One such potential target is the mycobacterial phosphatidylinositol phosphate synthase (M. tuberculosis PgsA1). PgsA1 catalyzes the conjugation of the 1’ hydroxyl group of D-myo-inositol-3-phosphate (ino-P) with a lipid tail of an acceptor substrate, cytidine diphosphate diacylglycerol (CDP-DAG), forming phosphatidylinositol phosphate (PIP). 1 D-myo-inositol-3-phosphate+CDP-DAG→PIP+CMP 2 PIP→PI+Pi PgsA1 belongs to the class I CDP-alcohol phosphotransferases (CDP-APs), integral membrane proteins that catalyze the formation of a phosphodiester bond to merge a CDP-alcohol and a second alcohol, releasing cytidine monophosphate (CMP). The M. tuberculosis PgsA1 was identified as a promising candidate for drug development, due to its essential role in growth and proliferation of the pathogen and differences between the Eukaryotic and mycobacterial PI biosynthesis pathways.

Here, we present the crystal structure of the full-length M. tuberculosis PgsA1 in absence of metals and substrates (apo) to 2.9 Å resolution and the 1.8 Å resolution structure of the CDP-DAG complex with a di-nuclear catalytic Mg2+ site. The electron density map does not contain any unexplained positive density in the vicinity of the protein active site that could correspond to the substrates or metal ions of PgsA1, therefore this structure is assigned to be in the apo state. In the apo structure the first 16 residues in chain A, and 15 in chain B, are disordered. In the metal-free form, the metal binding residues D68 and D71 appear to be almost completely disordered while D89 and D93 have better-defined electron density. Additionally, residues 149–151 (-FIE-), located on a loop connecting transmembrane helices 4 and 5, and eight C-terminal residues could not be traced in the electron density. The best binding energy was observed for binding mode #1 which was also the top solution in docking against both the CDP-DAG and the Mn-citrate complex structures. Both of the plausible binding modes were also observed when docking against the apo structure, albeit with worse binding energies and not representing the top solution.

>[2x]MSKLPFLSRAAFARITTPIARGLLRVGLTPDVVTILGTTASVAGALTLFPMGKLFAGACVVWFFVLFDMLDGAMARERGGGTRFGAVLDATCDRISDGAVFCGLLWWIAFHMRDRPLVIATLICLVTSQVISYIKARAEASGLRGDGGFIERPERLIIVLTGAGVSDFPFVPWPPALSVGMWLLAVASVITCVQRLHTVWTSPGAIDRMAIPGKGDR> MGWSLPKEKGLILCLWNKFCRWFHRRESWAQSRDEQNLLQQKRIWESPLLLAAKENNVQALYKLLKFEGCEVHQKGAMGETALHIAALYDNNEAAQVLMEAAPELVFEPMTSELYEGQTALHIAVINQNVNLVRALLARGASVSARATGSVFHYRPHNLIYYGEHPLSFAACVGSEEIVRLLIEHGADIRAQDSLGNTVLHILILQPNKTFACQMYNLLLSYDGGDHLKSLELVPNNQGLTPFKLAGVEGNIVMFQHLMQKRKHIQWTYGPLTSTLYDLTEIDSSGDDQSLLELIVTTKKREARQILDQTPVKELVSLKWKRYGRPYFCVLGAIYVLYIICFTMCCVYRPLKPRITNRTNPRDNTLLQQKLLQEAYVTPKDDLRLVGELVSIVGAVIILLVEIPDIFRLGVTRFFGQTILGGPFHVIIVTYAFMVLVTMVMRLTNSDGEVVPMSFALVLGWCNVMAFARGFQMLGPFTIMIQKMIFGDLMRFCWLMAVVILGFASAFYIIFQTEDPDELGHFYDYPMALFSTFELFLTIIDGPANYDVDLPFMYSITYAAFAIIATLLMLNLLIAMMGDTHWRVAHERDELWRAQVVATTVMLERKLPRCLWPRSGICGREYGLGDRWFLRVEDRQDLNRQRIRRYAQAFQQQDDLYSEDLEKDSGEKLVPR

TRPV6, a highly calcium-selective TRP channel, is overexpressed in endometrial cancers, leukemia, and carcinomas of the breast, prostate, colon, ovarian, and thyroid. TRPV6 has four subunits that form a transmembrane domain (TMD) with a central ion channel pore, an intracellular skirt domain enclosing a large cavity, and amphipathic TRP helices that run nearly parallel to the membrane and interact with both the TMD and the skirt. The TMD is composed of transmembrane helices S1–S6 and a re-entrant pore loop (P-loop) between S5 and S6. The first four transmembrane helices form a bundle to constitute the S1–S4 domain.

The strongest increase in potency of calcium uptake inhibition by 2-APB was observed for the mutant TRPV6*-Y466A. To shed light on the structural basis of this phenotype, we crystallized TRPV6*-Y466A in the presence and absence of 2-APB. In the absence of 2-APB, the C-terminal (cytoplasmic) part of S2 in TRPV6*-Y466A is splayed away from the binding pocket by ~4 Å relative to its position in TRPV6*-Y466A2-APB. In turn, 2-APB seems to glue the S2 helix back, perhaps by virtue of its tail amino group interaction with E402. Y466 in TRPV6* is highly conserved throughout the entire TRPV subfamily. In turn, a more loose binding pocket, such as the one observed in TRPV6*-Y466A, might cause reduction in TRPV6* affinity to the S1–S4 lipid and, as a result, increased affinity to 2-APB.>WSLRWRMQKSTTIAAIAGCSGAATFGGLAGGIVGCIAAGILAILQGFEVNWHNGGGGDRSNPV[2x];>[2x]GEATTIWGVGADEAIDKGTPSKNDL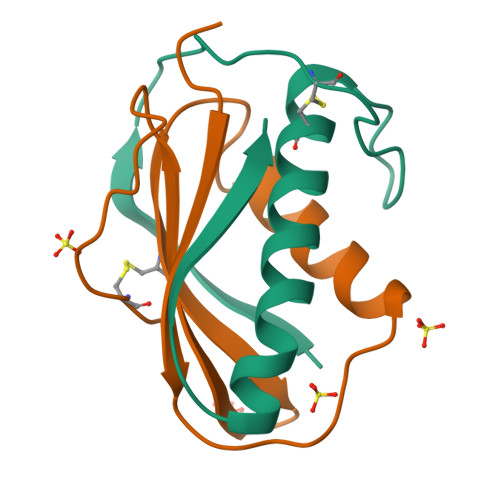QNMSADLAKNGFKGHQGVACSTVKDGNKDVYMIKFSLAGGSNDPGGSPCSDD[N-(2,4-DIAMINOPTERIDIN-6-YL)-METHYL]-DIBENZ[B,F]AZEPINE 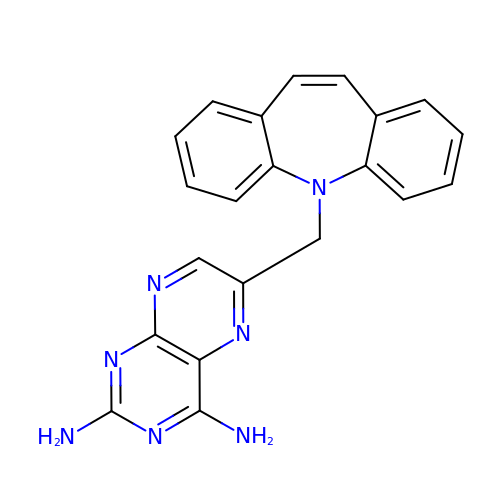| C21 H17 N7 | NXCCIJQEAKMFGW-UHFFFAOYSA-N METHYL 9-(BETA-D-TALOPYRANOSYLOXY)NONANOATE | C16 H30 O8 | 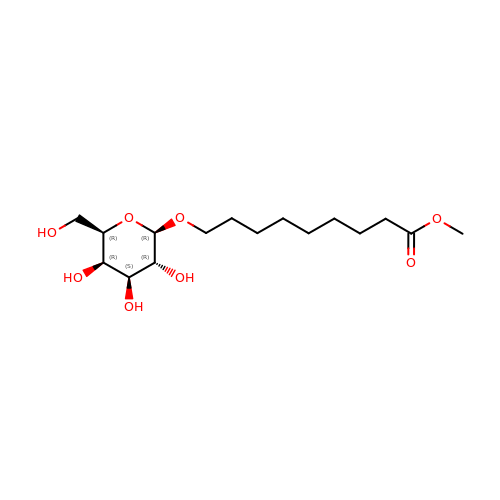ZJZBQHWSENWEMY-DZQJYWQESA-N>[2x]GSHMTLDRFVRIKYREDNEKVNRLVEILRELGLDCARTIEEKVDLQFDALRNLRENLKDDELFIKLVIANALVSYQLSGKGEDWWWEFSRYFSENPPEDIVEAYSSFLPNSKTNRRLVAGKLKRIERVEPFL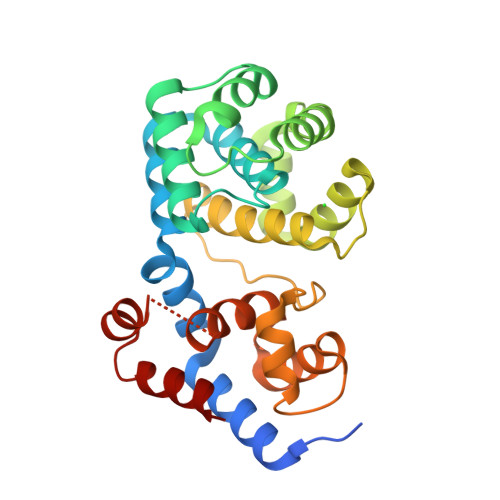SPLSISEIRDYYFNGMERLRDELARVMKAKRSAKTIVFAVKMFGYAGRIAFSAFVPYPMAIEIPDDVRINAYTKRFTSEPPVSFWGRIAEETGIPPLHIDSILWPVLGGKGEVLRRLKKHCGEKAERILELRDL> MNNGEGEVMDLRDIDLNLLVVFNQLLLDRSVSTAGEKLGLTQPAVSNSLKRLRTALNDDLFLRTSKGMEPTPYALHL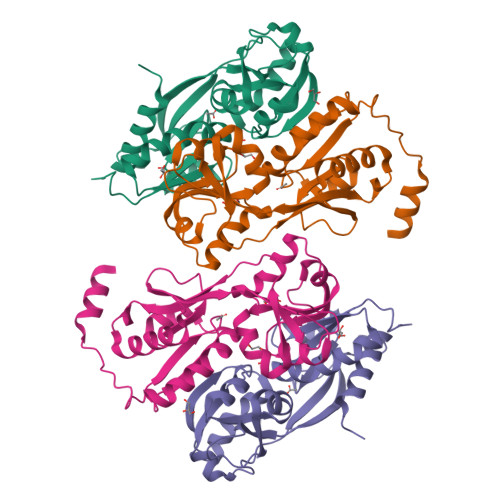AEPVIYALNTLQTALTTRDSFDPFASTRTFNLAMTDIGEMYFMPPLMEALAQRAPHIQISTLRPNAGNLKEDMESGAVDLALGLLPELQTGFFQRRLFRHRYVCMFRKDHPSAKSPMSLKQFSELEHVGVVALNTGHGEVDGLLERAGIKRRMRLVVPHFIAIGPILHSTDLIATVPQRFAVRCEVPFGLTTSPHPAKLPDIAINLFWHAKYNRDPGNMWLRQLFVELFSEAHHHHHH;> MNNGEGEVMDLRDIDLNLLVVFNQLLLDRSVSTAGEKLGLTQPAVSNSLKRLRTALNDDLFLRTSKGMEPTPYALHLAEPVIYALNTLQTALTTRDSFDPFASTRTFNLAMTDIGEMYFMPPLMEALAQRAPHIQISTLRPNAGNLSEDMESGAVDLALGLLPELQTGFFQRRLFRHRYVCMFRKDHPSAKSPMSLKQFSELEHVGVVALNTGHGEVDGLLERAGIKRRMRLVVPHFIAIGPILHSTDLIATVPERFAVRCEVPFGLTTSPHPAKLPDIAINLFWHAKYNRDPGNMWLRQLFVELFSEAHHHHHH> ANNLGSKLLVGYWHNFDNGTGIIKLKDVSPKWDVINVSFGETGGDRSTVEFSPVYGTDADFKSDISYLKSKGKKVVLSIGGQNGVVLLPDNAAKDRFINSIQSLIDKYGFDGIDIALESGIYLNGNDTNFKNPTTPQIVNLISAIRTISDHYGPDFLLSMAPETAYVQGGYSAYGSIWG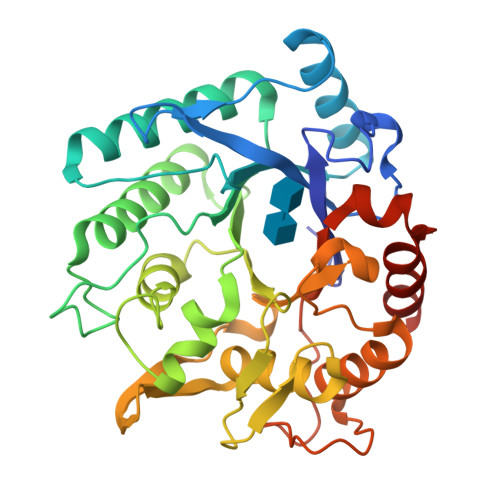AYLPIIYGVKDKLTYIHVQHYNAGSGIGMDGNNYNQGTADYEVAMADMLLHGFPVGGNANNIFPALRSDQVMIGLPAAPAAAPSGGYISPTEMKKALNYIIKGVPFGGKYKLSNQSGYPAFRGLMSWSINWDAKNNFEFSNNYRTYFDGLSLQK>[4x]SLVELGKMILQETGKNPAKSYGAYGCNCGVLGRGKPKDATDRCCYVHKCC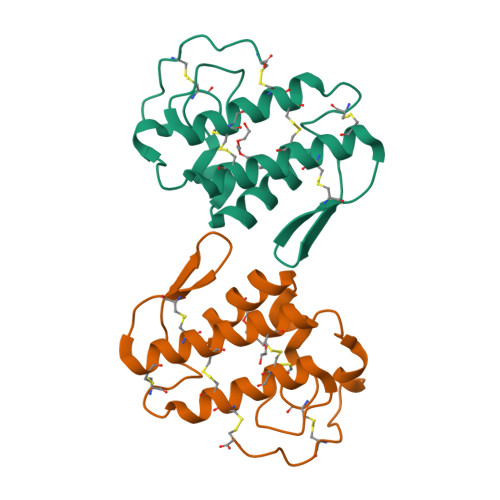YKKLTDCDPKKDRYSYSWKDKTIVCGENNSCLKELCECDKAVAICLRENLDTYNKKYRNNHLKPFCKKADPC>[5x]GQDMVSPPPPIADEPLTVNTGIYLIECYSLDDKAETFKVNAFLSLSWKDRRLAFDPVRSGVRVKTYEPEAIWIPEIRFVNVENARDAAVVDISVSPDGTVQYLERFSARVLSPLDFRRYPFDSQTLHIYLIVRSVDTRNIVLAVDLEKVGKNDDVFLTGWDIESFTAVVKPANFALEDRLESKLDYQ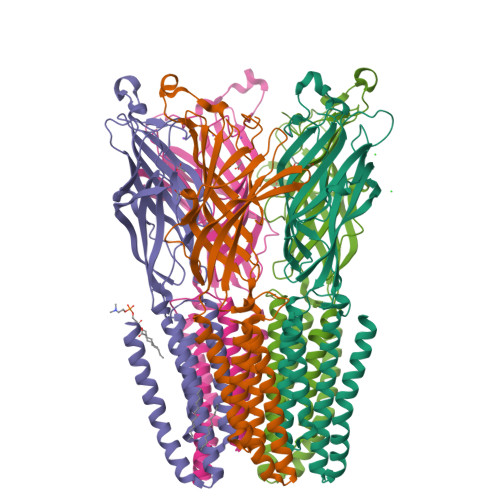LRISRQYFSYIPNIILPMLFILFISWTAFWSTSYEANVTLVVSTLIAHIAFNILVETNLPKTPYMTYTGAIIFMIYLFYFVAVIEVTVQHYLKVESQPARAASITRASRIAFPVVFLLANIILAFLFFGF> MFIINSDFHRGNMEQYQKAQKLSFDPAELLRTSLNVGDIVLLKQCTSELTMCVNLPQSTTDPRYTFAKKDGTLVYAMKNSVILRIPKDLPEEVNQLLKRESNHPYQKIGTIKNSSNETEILPVLTRQLIVSFTLATFTKFAWTQLPIVLKKLELIHRYLQDSRGSKHVNFMSLVRIIKNLNIKEATDAINGDAYVRKVIDESMSVVNKSIDPTTLLATYWGVREQQQNNLWGSVYTNTALLSPTTVAVLPLKKAHLFYQEVITRLESNDYQEIKAFAKLVNDKDYHSIAKRYDYIRTLLNDYAAGNIEENAVLTTIISKIFRHIDMYRDQDVTRSLCGKLLVEISPQSNSSNFILGNWDLNIPKSSGISSVEQKLYDTAMPTIVSDTDRYDFGDMPVFCIDSEDAHEINDGISIEELDGVRSRIHIHIADPAGLFPESFDYTKSGISDDVLRV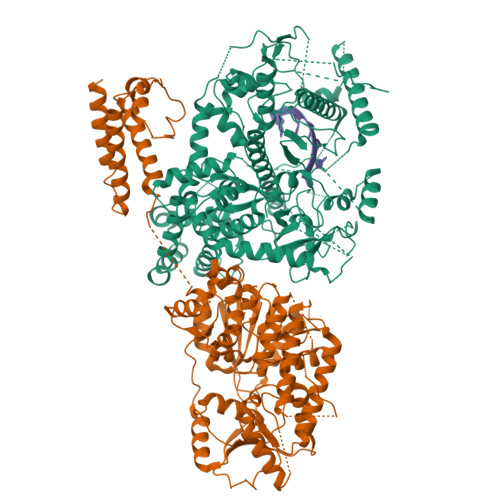SLKRAFTTYLPDLVVPMLPKSFCNRADLGKHDRKTETISFSFELVNKEDGGLHVDYDTFQVRLGIVSNFPKVTYDKVDSILNGDDNSLPSKQKKQLELLHTLATKLLHKRIHDDNAVVFGDGFNKGLVSLSPDDDGELCIPTFYDQSQTKSTLLVSEFMILTNKLCAAFFQENKIPGVYRCYNGLNLGNQAKAQFELLKENIKLGKLPSLKDITKISSQLSSSFYSPFPLPHKMIGNTAYLTVTSPMRRGPDLINHLQLHRFLKKLPLCFKQEYLDQYVWSFQARADILKIFQRHSSTYWTLKHLEQSGTKTHDVIVTSVPQNGTVNCLFPEYSYARGTLKLDPAMKKIPRIGDTIRHCKVESIHPLDGILTLTHVNRK;> MIYTTDKEFKKNLENALAHVYSTQIENSAPDQVEFRKVAWLRLKDMLYNQLLDKNLPAKINGYDPGLMETISPTQPQHIIPHLVKMNKIDQLIWKKITGKTEGVTKYEQFQYLLSSYYDCILNQEIIPSMLNTGTDDSVHSVDFSNPAEWFPEARKIRRHIIMHVGPTNSGKTFRSLQKLKAADRGYYAGPLRLLAREVYEKFKHENVRCNLLTGEEVIKDLDEMGNEANLTSGTIEMIPLNQNFDVVVLDEIQMMADLDRGWAWTNALLGAKAKEVHCCGEASTIPLIKKIVEMTGDKLTINEYERMGKLVVEEEALTKGYHSLKKGDCVVAFSKKAILDLKLEIEKKTELKAAVIYGSLPPETRVKQANLFNSGEFDILIASDAIGMGLNLSIDRVVFTTSKKFDGRDMVDMTSSAIKQIGGRAGRFKQNIHDNGELPVGYITAVKPNVLKAVREAINAPIEYLTSATTWPTDEICTHVMTRFMPGTTCKTLLETIAADIEQSSNKLFQICDLKARMSAIEIIDSMEDITFSDKLRLSNAPLKDFPLVKAAFKKFCDTIARGHTRGLLSYRFPFDILNLKYIYTEKHGLEEYEALYNIIMLFFWLSNRYPNYFIDQESASELKNFCEMIIFEKIDHLKRNPY> MGSSHHHHHHGSQQSQPNVLVFYVDDLRAELGCYGSKTAITPNIDKLATEGVQFNKAYVQQAICAPSRMSTLTGLRPETLGIYSIFTPLRSVHKDVVSVPQLFKENGYKTVSIGKVYHHGTDDKNQWTNYFTKEPNTYNKPENIALLEQFKKEGKKANGPAFENADVADEAYKDGRAAKYAVETLKKLKNDKFIMFVGFSKPHLPFNAPKKYWDLYDKNNFEIPERKKPENMYRLALTNWGELKGYHGIPNDVEYLDDNLTRDLIHGYHASISYV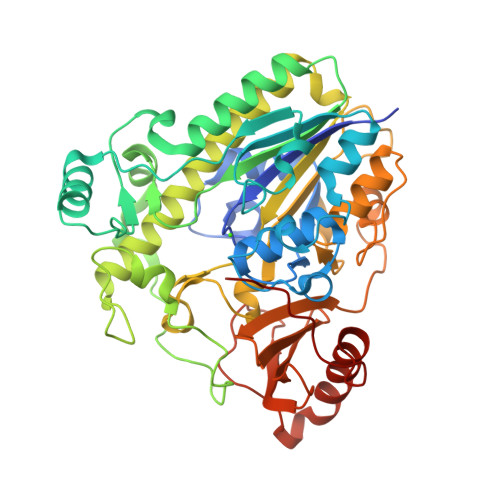DAQVGKVMEALEALGLRKNTTVIFMSDHGYKIGEYGAWCKHSNEEIDVRVPLIVSRETSYKGRVAGKTSDALVENVDIFPTLVELCGLEGPKTDGKSILQVIDRPNTPWDQVATAVYARGKNIMGCTATDGEWRYTEWRDAKTQDILGAELYEHKNSLLSFKNLSGNTKYKKEEARMKGLLETQFPRNQGPFLQHDTPRN>MSKQQPTQFINPETPGYVGFANLPNQVHRKSVKKGFEFTLMVVGESGLGKSTLINSLFLTDLYPERVIPGAAEKIERTVQIEASTVEIEERGVKLRLTVVDTPGYGDAINCRDCFKTIISYIDEQFERYLHDESGLNRRHIIDNRVHCCFYFISPFGHGLKPLDVAFMKAIHNKVNIVPVIAKADTLTLKERERLKKRILDEIEEHNIKIYHLPDAESDEDEDFKEQTRLLKASIPFSVVGSNQLIEAKGKKVRGRLYPWGVVEVENPEHNDFLKLRTMLITHMQDLQEVTQDLHYENFRSERLKRGGRKVENED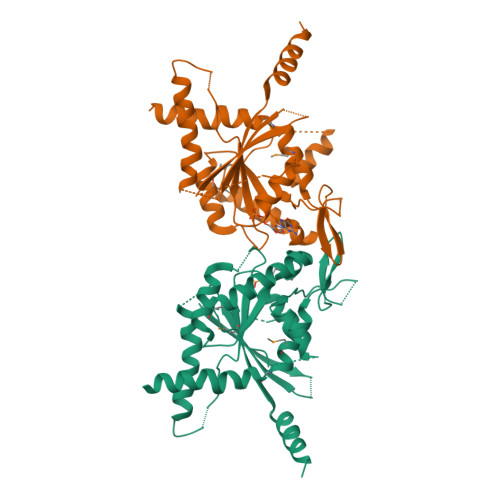[2x]>[4x]MTLGTNQVSKTHSFMTVSLIELWERFGYYGMQALIVYFMVQRLGFDDSRANLVWSACAALIYVSPAIGGWVGDKILGTKRTMLLGAGILSVGYALMTVPTENTWFMFSALGVIVVGNGLFKPNAGNLVRKIYEGDDSKIDSAFTIYYMAVNVGSTFSMLLTPWIKDYVNAQYGNEFGWHAAFAVCC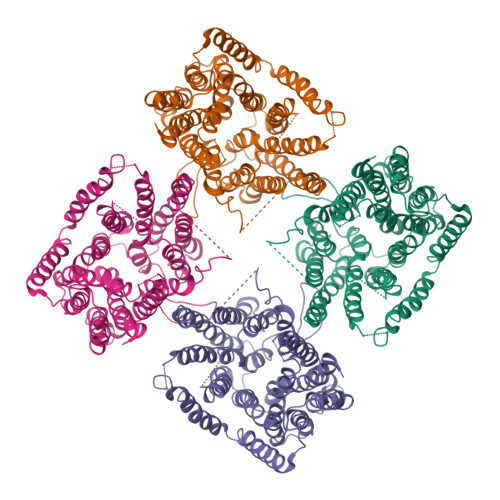VGILVGLGNYALMHKSLANYGSEPDTRPVNKKSLAIVLALAALSVVASAIILEYEDVARVFVYAAGVAVLGIFFHLIRTSEPSERAGLIAALILTVQTVFFFIFYQQMSTSLALFALRNVDWDFQVFGTHLWTWSPAQFQALNPIWIMVLSPVLAWSYSWAGRNNKDFSIAAKFALGFAVVAIGFFIYGFAGQFAVNGKTSSWVMIWGYASYSLGELLVSGLGLAMIARYVPARMGGFMMGAYFVASGISQYLGGVVANFASVPQDLVDPLQTLPVYTNLFNKLGVAAVVCTIIALAVLPLMRRLTESHHAHSSIENNAAASLRDVKAEQLESSGENLYFQ>HHHHHHHHHHSSGHIDDDDKHMNYLSPAKIDSLFSAQKAYFATRATADVGFRKQSLERLKEAVINNKEALYSALAEDLGKPKDVVDLAEIGAVLHEIDFALAHLDEWVAPVSVPSPDIIAPSECYVVQEPYGVTYIIGPFNYPVNLTLTPLIGAIIGGNTCIIKPSETTPETSAVIEKIIAEAFAPEYVAVIQGGRDENSHLLSLPFDFIFFTGSPNVGKVVMQAAAKHLTPVVLELGGKCPLIVLPDADLDQTVNQLMFGKFINSGQTXIAPDYLYVHYSVKDALLERLVERVKTELPEINSTGKLVTERQVQRLVSLLEATQGQVLVGSQADVSKRALSA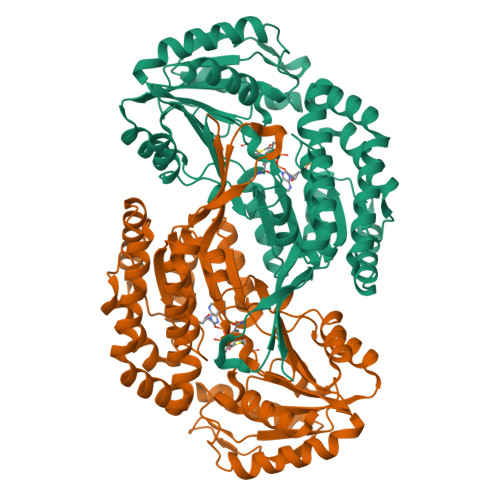TVVDGVEWNDPLMSEELFGPILPVLEFDSVRTAIDQVNKHHPKPLAVYVFGKDMDVAKGIINQIQSGDAQVNGVMLHAFSPYLPFGGIGASGMGEYHGHFSYLTFTHKKSVRIVP[2x]>[8x]MRGSHHHHHHENLYFQGSMLIDLITSYRKTAAIYTFVDAGLSIHFKNGDYVDINKLASQYGIDYSRLNRLCDFLIEIGVLVSSDHGVALSEECSALADPNSVEFLTVKYEINSEHWDSWLMYPKSLLENNGKSAFEMVHGKSFFEHLDSNKGLKSDFDALMSKYTNKIIKELLVIYDFD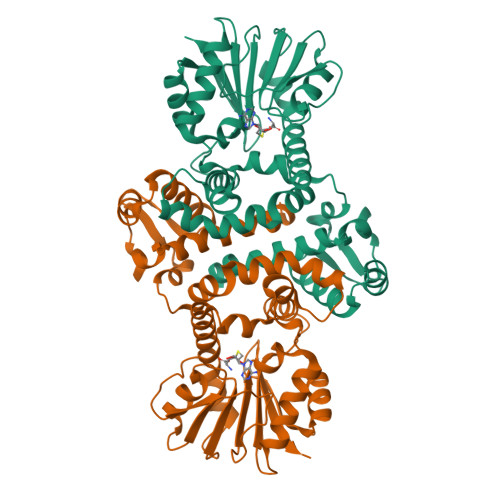KHNRILDLGGGDGELLIRISEQVKGKDYTVLDRYNEVPISEGINFIKGDFFKPIPTGYDLYILKNVLNNWPDNDAISILKNCREAMDNNATLLIITLMKKPQSLVVKSVDILMDMLFSAKQRYLSEFEDIANQAGLVIRHYKDLDEIFSLIELKVK HSPB7 is a member of the small Heat-Shock Protein (sHSP) family, and is expressed specifically in heart and skeletal muscle. Though it shares the common architecture of sHSPs (an α-crystallin domain, ACD, flanked by N- and C-terminal regions), HSPB7 is unusual as it has been observed to be oligomerisation incompetent. FLNC interacts with HSPB7, also known as cardiovascular heat-shock protein (cvHSP), via d2417–20. Our work therefore shows, structurally, how HSPB7 acts as a specific molecular chaperone that regulates FLNC dimerisation.

To investigate why none of the HSPB7 constructs dimerise to an appreciable extent, we turned to X-ray crystallography. We undertook crystallisation trials on HSPB7ACD and HSPB7ΔN, but did not obtain any protein crystals. We speculated that this might be due to a solvent-accessible cysteine (C131) leading to non-specific intermolecular interactions during crystallisation, and hence generated the C131S mutant of both constructs. Of these, HSPB7ACDC131S returned good crystals, which diffracted to 2.2 Å resolution; the structure was solved by molecular replacement in the P41212 space group. B The Ig-fold is very similar to that of other sHSP ACDs: it contains six β strands, with a groove between β4 and β8 and an extended “β6 + 7” strand. The monomers within the asymmetric unit contact each other through crystallographic interfaces between neighbouring anti-parallel β4 and β6 + 7 strands that form long chains of monomers in the crystal. The lack of a head-to-head dimer in the crystal form is different to most sHSP ACD structures that have been determined, but is consistent with our native MS data that showed monomers to be the dominant form in solution. A rationale for this might be that the β6 + 7 strand is shorter in HSPB7 compared to that found in the canonical human sHSPs; in particular it is missing charged amino acids at positions 118 and 129 that form inter-monomer salt bridges in HSPB1 and HSPB5. These differences likely act to reduce the strength of a putative anti-parallel interaction of two β6 + 7 strands (as per the canonical metazoan sHSP dimer), with the result that HSPB7 exists primarily as a monomer.

>[3x]GSGNIKTLGDAYEFAVDVRDFSPEDIIVTTSNNHIEVRAEKLAADGTVMNTFAHKSQLPEDVDPTSVTSALREDGSLTIRARRHPHT>[4x]GAMDPLGLQDFDLLRVIGRGSYAKVLLVRLKKTDRIYAMKVVKKELVNDDEDIDWVQTEKHVFEQASNHPFLVGLHSCFQTESRLFFVIEYVNGGDLMFHMQRQRKLPEEHAR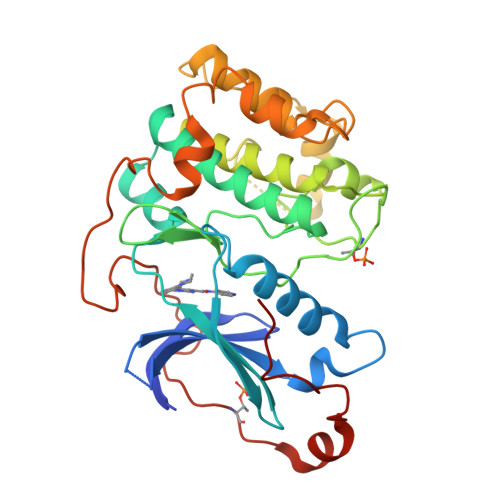FYSAEISLALNYLHERGIIYRDLKLDNVLLDSEGHIKLTDYGMCKEGLRPGDTTSTFCGTPNYIAPEILRGEDYGFSVDWWALGVLMFEMMAGRSPFDIVGSSDNPDQNTEDYLFQVILEKQIRIPRSLSVKAASVLKSFLNKDPKERLGCHPQTGFADIQGHPFFRNVDWDMMEQKQVVPPFKPNISGEFGLDNFDSQFTNEPVQLTPDDDDIVRKIDQSEFEGFEYINPL> GSHMDNQCTVQVRLELGHRAQLRKKPTTEGFTHDWMVFVRGPEQCDIQHFVEKVVFWLHDSFPKPRRVCKEPPYKVEESGYAGF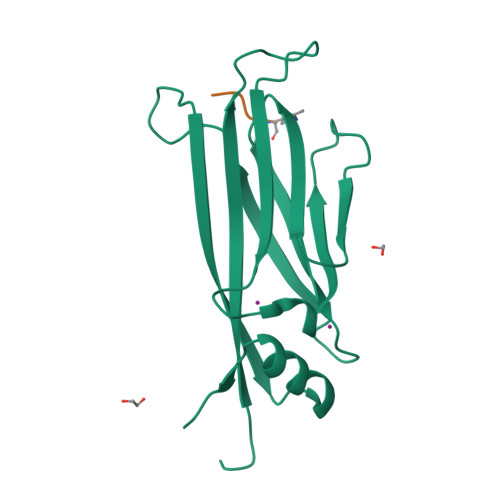IMPIEVHFKNKEEPRKVCFTYDLFLNLEGNPPVNHLNHLRCEKLTFNNPTTEFRYKLLRAGGVMVMPEGAHHHHHH;> AARK> KHNMKAFLDELKAENIKKFLYNFTQIPHLAGTEQNFQLAKQIQSQWKEFGLDSVELAHYDVLLSYPNKTHPNYISIINEDGNEIFNTSLFEPPPPGYENVSDIVPPFSAFSPQGMPEGDLVYVNYARTEDFFKLERDMKINCSGKIVIARYGKVFRGNKVKNAQLAGAKGVILYSDPADYFAPGVKSYPDGWNLPGGGVQRGNILNLNGAGDPLTPGYPANEYAYRRGIAEAVGLPSIPVHPIGYYDAQKLLEKMGGSAPPDSSWRGSLKVPYNVGPGFTGNFSTQKVKMHIHSTNEVTRIYNVIGTLRGAVEPDRYVILGGHRDSWVFGGIDPQSGAAVVHEIVRSFGTLKKEGWRPRRTILFASWDAEEFGLLGSTEWAEENSRLLQERGVAYINADSSIEGNYTLRVDCTPLMYSLVHNLTKELKSPDEGFEGKSLYESWTKKSPSPEFSGMPRISKLGSGNDFEVFFQRLGIASGRARYTKNWETNKFSGYPLYHSVYETYELVE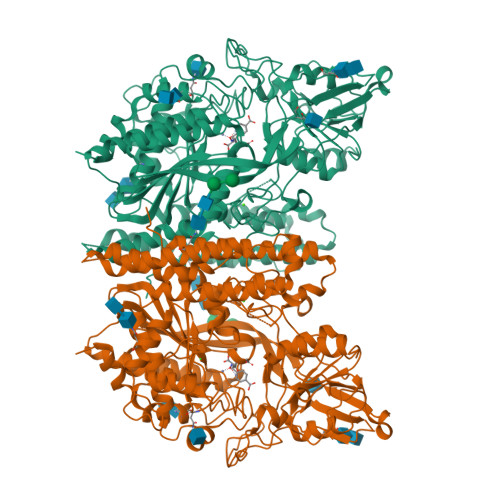KFYDPMFKYHLTVAQVRGGMVFELANSIVLPFDCRDYAVVLRKYADKIYSISMKHPQEMKTYSVSFDSLFSAVKNFTEIASKFSERLQDFDKSNPIVLRMMNDQLMFLERAFIDPLGLPDRPFYRHVIYAPSSHNKYAGESFPGIYDALFDIESKVDPSKAWGEVKRQIYVAAFTVQAAAETLSEVA>[2x]MYDYIIVGSGLFGAVCANELKKLNKKVLVIEKRNHIGGNAYTEDCEGIQIHKYGAHIFHTNDKYIWDYVNDLVEFNRFTNSPLAIYKDKLFNLPFNMNTFHQMWGVKDPQEAQNIINAQKKKYGDKVPENLEEQAISLVGEDLYQALIKGYTEKQWGRSAKELPAFIIKRIPVRFTFDNNYF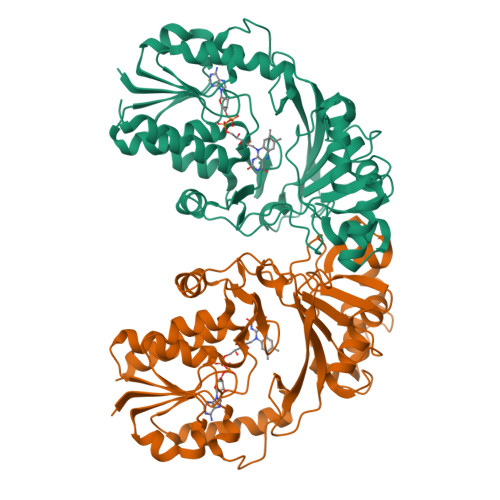SDRYQGIPVGGYTKLIEKMLEGVDVKLGIDFLKDKDSLASKAHRIIYTGPIDQYFDYRFGALEYRSLKFETERHEFPNFQGNAVINFTDANVPYTRIIEHKHFDYVETKHTVVTKEYPLEWKVGDEPYYPVNDNKNMELFKKYRELASREDKVIFGGRLAEYKYYDMHQVISAALYQVKNIMSTD> SMEMPVDRILEAELAVEQKSDQGVEGPGGTGGSGSSPNDPVTNICQAADKQLFTLVEWAKRIPHFSSLPLDDQVILLRAGWNELLIASFSHRSIDVRDGILLATGLHVHRNSAHSAGVGAIFDRVLTELVSKM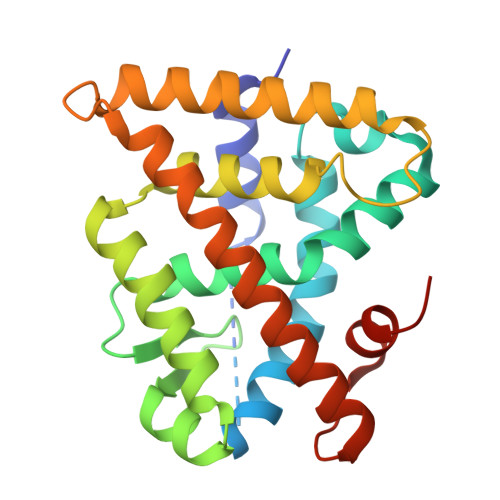RDMRMDKTELGCLRAIILFNPDAKGLSNPSEVEVLREKVYASLETYCKQKYPEQQGRFAKLLLRLPALRSIGLKCLEHLFFFKLIGDTPIDTFLMEMLEAPHQLA> GGAAUCUCGCCCGAUGUUCGCAUCGGGAUUUGCAGGUCCAUGGAUUACACCAUGCAACGCAGACCUGUAGAUGCCACGCUAGCCGUGGUGAGGGUCGGGUCCAGAUGUCAUUCGACUUUAACGCGCCUAAGCGUUGAAGGCGUGUUAGAGCAGAUAGUUCGCUAUCUGGGGAGCCUGUUCGCAGGCUCAGGAGCCUUCGGGCUCCUAGCGCUAUUACCCCGGACACCACCGGGCAGACAAGUAAUGGUGCUCCUCGAAUGACUUCUGUUGAGUAGAGUGUGGGCUCCGCGGCUAGUGUGCACCUUAGCGGUGAAUGUCUGACACCGUUAA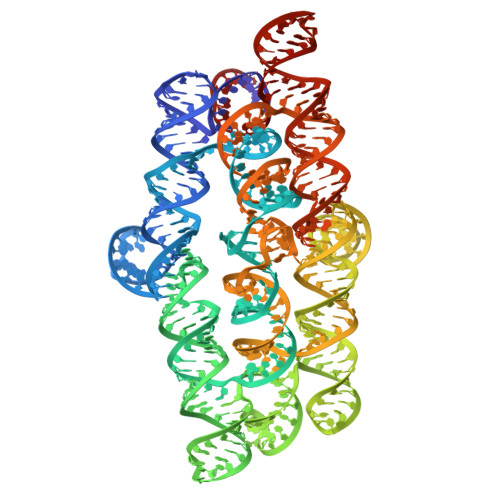GGUGGUUACUCUUCGGAGUAACGCCGAGAUUCC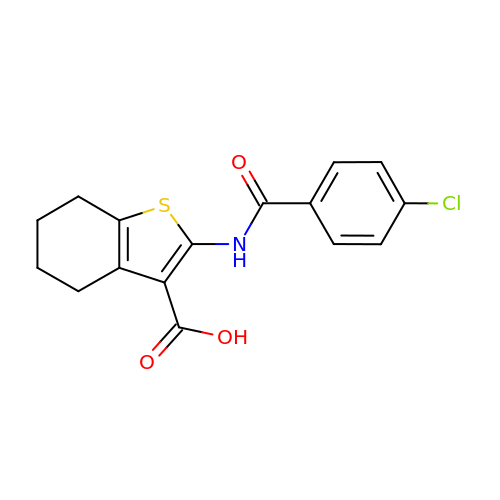2-(4-chlorobenzamido)-4,5,6,7-tetrahydro-1-benzothiophene-3-carboxylic acid | C16 H14 Cl N O3 S | DUJFDTGMUKWELI-UHFFFAOYSA-N> GPGSNEFYLKT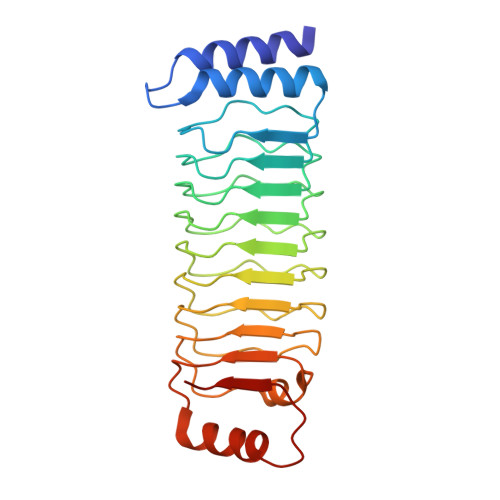WSEWEKNGTPGEQRNIAFNRLKICLQNQEAELNLSELDLKTLPDLPPQITTLEIRKNLLTHLPDLPPMLKVIHAQFNQLESLPALPETLEELNAGDNKIKELPFLPENLTHLRVHNNRLHILPLLPPELKLLVVSGNRLDSIPPFPDKLEGLALANNFIEQLPELPFSMNRAVLMNNNLTTLPESVLRLAQNAFVNVAGNPLSGHTMRTLQQITTGPDYSGPRIFFSMG(~{Z})-2-cyano-~{N},~{N}-dimethyl-3-[5-[3-[(1~{S},2~{R})-2-methylcyclohexyl]-3,5,8,10-tetrazatricyclo[7.3.0.0^{2,6}]dodeca-1,4,6,8,11-pentaen-4-yl]furan-2-yl]prop-2-enamide 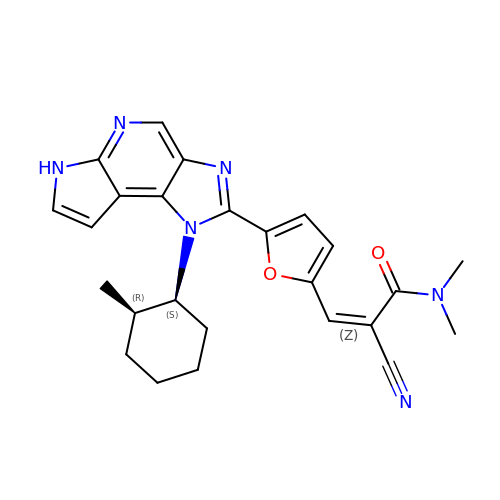| C25 H26 N6 O2 | LVVYJCDRPPCFEQ-YXEVWGHGSA-N6-((4-chlorophenyl)thio)-[1,2,4]triazolo[4,3-b]pyridazin-3(2H)-one | 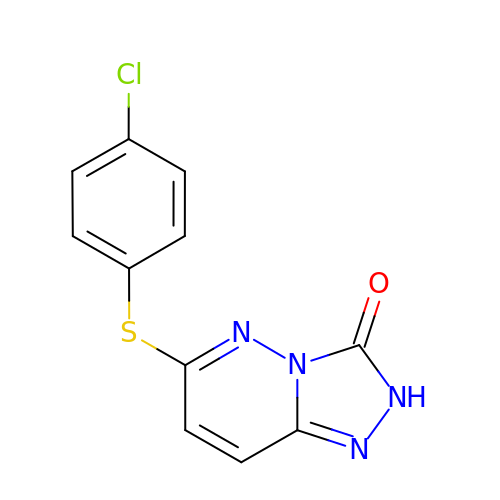C11 H7 Cl N4 O S | YMDYCZLBRZYSTF-UHFFFAOYSA-N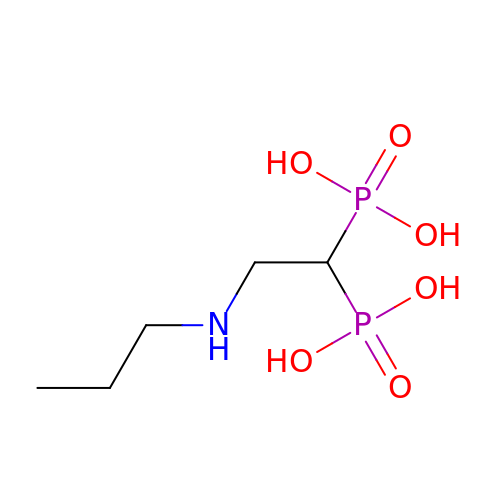[2-(propylamino)ethane-1,1-diyl]bis(phosphonic acid) | C5 H15 N O6 P2 | YFFJUBPLIKXHAO-UHFFFAOYSA-N> GA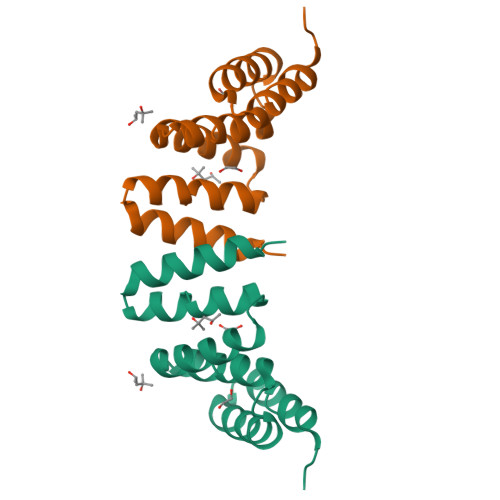MDPGNSAEAWYNLGNAYYKQGDYDEAIEYYQKALELYPNNAEAWYNLGNAYYKQGDYDEAIEYYQKALELYPNNAEAWYNLGNAYYKQGDYDEAIEYYQKALELYPNNAEAKQNLGNAKQKQG> MNGPQTRESLANEIWRACDIMRRDNN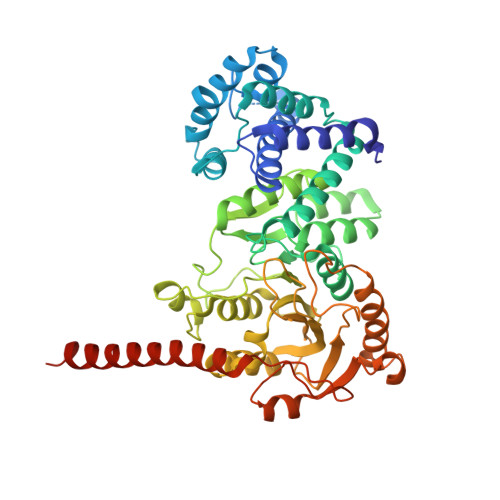CTGIMEYVEHLAWLLFLRFLDAQEEEWEAQAQIAGRPYTPIIDSEYRWRHWATKDWPADELLAFVHGRLIPYLRSLGGDPLRETIRSLFSERNVIVCASGYNLKDVIQIVNEINFHSQDDIFTVSQVYEELLRRLGNENRLAGEFYTPRPVVRFVVELVDPQIGEAVYDPACGTCGFLVEAYLWMKQKERTIEDHRILQERTFFGQEKKPVPAFLGLVNMMLHGVTVPRVMRRNTLEENIRNVSERFDVVVTNPPFGGTEGRHIQQNFPIQSNATELLFLQHIMKKLKPRDGARCGMVVPEGTLFRGGAFAEVKRDLLEQFNLHTVVSLPPGTFAPYSDVKTALIFFERPGPTKEIWYYELPLPEGLKKFSKGNPIQDEHFEEARKLWRGWDAYRKGLGPVEACLSERSWIVPVEEVKKRGYDLTARNPNRSGGEELPSPVEIVAGLLEKEREILSIMEELSELLENEKGNSSRKNDEEEE> MQQSVCRARPIWWGTQR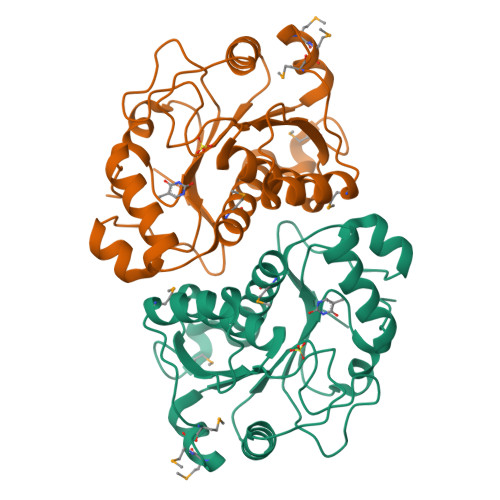RGSETMAGAAVKYLSQEEAQAVDQELFNEYQFSVDQLMELAGLSCATAIAKAYPPTSMSKSPPTVLVICGPGNNGGDGLVCARHLKLFGYQPTIYYPKRPNKPLFTGLVTQCQKMDIPFLGEMPPEPMMVDELYELVVDAIFGFSFKGDVREPFHSILSVLSGLTVPIASIDIPSGWDVEKGNPSGIQPDLLISLTAPKKSATHFTGRYHYLGGRFVPPALEKKYQLNLPSYPDTECVYRLQHHHHHH> MIGGLFIYNHKGEVLISRVYRDDIGRNAVDAFRVNVIHARQQVRSPVTNIARTSFFHVKRSNIWLAAVTKQNVNAAMVFEFLYKMCDVMAAYFGKISEENIKNNFVLIYELLDEILDFGYPQNSETGA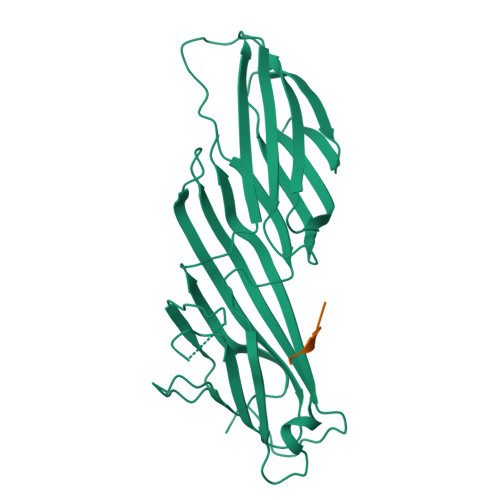LKTFITQQGIKSQHQTKEEQSQITSQVTGQIGWRREGIKYRRNELFLDVLESVNLLMSPQGQVLSAHVSGRVVMKSYLSGMPECKFGMNDKIVIEKQGKGTADETSKSMEQKLISEEDLGKQSIAIDDCTFHQCVRLSKFDSERSISFIPPDGEFELMRYRTTKDIILPFRVIPLVREVGRTKLEVKVVIKSNFKPSLLAQKIEVRIPTPLNTSGVQVICMKGKAKYKASENAIVWKIKRMAGMKESQISAEIELLPTNDKKKWARPPISMNFEVPFAPSGLKVRYLKVFEPKLNYSDHDVIKWVRYIGRSGIYETRC;> QYKSILQE>[4x]MHSLMKPTREPQINLFKKSNPYKAKVISNVLLTPETGTGKRPKKEGEALVHRIVLAIDHSAYPYVIGQSGGVIPPGEDPEKKAKGLADVGYTVRLYSIASPSYSFGMKEDNIEFIIKRDNIYDENGNIQFKGVCSNYMCDLKPGDEVTMTGPSGKKFLLPNTDFSGDIMFLATGTGIAPFIGMSEELLEHKLIKFTGNITLVYGAPYSDELVMMDYLKGLESKHKNFKLITAISREEKNSFDGGRMYISHRVREQAEAVKKILNGGGRFYICGGPKGMEKGVIEEIQKISGNTGTYEEFKHHLEGAHQLFVETY

Ferredoxin-NADP(H) reductases (FNRs) are flavoenzymes that catalyze electron transfer between NADP(H) and the iron-sulfur protein ferredoxin (Fd) or flavin mononucleotide-containing flavodoxin. Leptospira interrogans FNR (LepFNR) displays low sequence identity with plant (34% with Zea mays) and bacterial (31% with Escherichia coli) FNRs. Crystal structures of LepFNR reveal a typical plastidic type reductase, analogous in its folding architecture to the enzymes found in plant and cyanobacteria, in spite of displaying an important divergence at primary structure level. Overall topology of the LepFNR molecule has the canonical FNR fold, which consists of two well defined domains, although several unique structural features were found in LepFNR 3D structure.

The quality of the LepFNR crystal structure, refined to 2.4 Å resolution, is fine as judged by stereochemical and refinement parameters. Crystal structure analysis reveals that unlike in usual prokaryote FNRs, LepFNR accommodates the FAD molecule in an extended conformation between the two enzyme domains. The flavin group of FAD is tightly bound to FNR binding cleft through strong hydrogen bonds. The main chain atoms of Ser97, Ile115, Lys117 and Leu95 interact directly with flavin moiety creating the core of the binding site. Cys134, Arg94, Ser135 and Val133 are at hydrogen bonding distances to pyrophosphate group strongly anchoring it to LepFNR cleft. Adenosine ribose is also involved in strong hydrogen bond interaction with Asp119 as judged from a short 2.71 Å length of this bond. The phenol ring of the carboxyl terminal tyrosine (Tyr314) and the flavin group are practically coplanar maximizing π-orbital overlapping, as have been observed in all plastidic class FNRs, resulting in a large portion of the isoalloxazine moiety shielded from the bulk solution. Surprisingly, in LepFNR FAD acquired a different conformation in which its adenine moiety interacts with Phe130. LepFNR, on the other hand, exhibits higher sequential identity with plant FNRs and does not contain cysteine residues in the position required to form the intermolecular disulfide bridge. This analysis strongly suggests that metal mediated LepFNR dimerization, observed in the crystal structure, is induced by crystallization effects and do not represent a physiologically relevant oligomeric state of the protein.> NNDDPVENFVESTLKEVLVVPDTKPSGPQHTTKPSILGAMEIGASSNATPESTIETRYVYNTNTNAEADVEMFLGRSALWGKVTLTRQYAKWEINFQEQAHIRKKFEFFTYLRFDMEVTIVTNNKGLMQIMFVPPGIDHPETHDDRKWD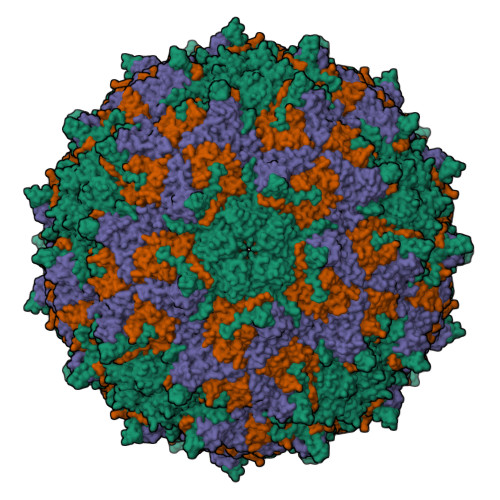SASNPSVFFQPKSGFPRFTIPFTGLASAYYMFYDGYDKPKGSDNNEYGIAPTNDMGLLCFRTLDNSGGNDVKIYVKPKHITAWVPRPPRATQYTHKYSTNYHYKPNSSGPDEHVLKDRHFIKTRPLISSA;> GLPTRLPSGSQQFMTTEDEQSPNILPGFHPSKKIHIPGMITNVMHMARVDSFIPINNIQGEVGKVSMYYITVTKKTVTERILVLPLEMSNTLFATTLLGEVLNYYANWSGSITITFMCVCDAFSTGKFLVAYTPPGGKLPEDRKQAMLGVHIIWDLGLQSSCTIVVPWISSGFYRRTKADSFTHGGYVSLWYQTAFVPPVSGGTGSILATCSACPDMSVRMLRDSPMMEQKNELQ;> SPSVEACGYSDRLKQITIGNSTITTQDSLHTVLAYGEWPTYLSDIDATSVDKPTHPETSADRFYTLDSVEWQVGSHGWWWKLPDALKDMGVFGQNMYYHSMGRSGFIIHTQCNATKFHSGALIVAVIPEHQLAYVGGVKVNVGYDHTHPGQSGHQIRGPSQSNDRSGGKPDEDPLFNCNGTLLGNITIFPHQIINLRTNNSSTIVVPYINCVPMDNMLKHNNLSLVIIPLVPLRPGSSGINSVPITVTIAPYKSEFSGAMEAQRQ;> GAQVSRQNNGTHENGVTASNGSVIKYFNINYYKDSASSGLSRQDFSQDPSKFTQPLVDTLTNPALM A-1(L) is a Myoviridae cyanophage isolated in 1970s9 that specifically infects the model cyanobacterium Anabaena sp. PCC 7120. Using cryo-electron microscopy (cryo-EM), we solved the structure of A-1(L) tail machine, which consists of three parts: a 205-Å-long neck, a 1045-Å-long contractile tail with a complicated baseplate, and six pairs of tail fibers. The dodecameric gp2 portal, the pentadecameric gp5 and the hexameric gp7 sequentially constitute the neck of A-1(L), to which five neck fibers are attached. The long and contractile tail of A-1(L) contains 24 rings of gp10 hexamers that form the tube, surrounded by the sheath of 24 helically stacked gp9 hexamers.

Moreover, docking of tail to the neck is accomplished via direct interactions: Loopβ4-β5 (residues Gly55-Thr65) of one gp7 subunit and antiparallel β4′-β5′ hairpin of neighboring subunit interact with Loopα1-β1 (residues Ile15-Val34) and Loopβ5-β6 (residues Leu135-Trp152) of one terminator/gp8 subunit, respectively. In detail, the ring formed by Loopα4-α5 (residues Ile83-Tyr99) of 15 gp5 subunits is hooked by six long α1 helices (residues Met1-Leu25) at the N-terminus of gp7, whereas Loopα1-α2 (residues Leu20-Glu30) of three gp5 subunits tightly interact with the Loopβ5-β6 (residues Thr70-Lys75) of trimeric gp82N. In contrast to the initiation with two separate proteins, the termination of the tube and sheath is fulfilled by a same terminator. Each terminator subunit simultaneously interacts with two tube subunits via Loopβ3-β4 (residues Thr58-Gln71) and β5 (residues Thr125-Leu135), and one sheath subunit via a protruding β7-β8 hairpin (residues Asn202-Ile240), which disrupts the inter-ring interfaces of the tube and sheath, and eventually terminates the extension of tail. Notably, the A-1(L) terminator is structurally different from the previously reported ones in the tailed phages and eCISs. The tube and sheath start from the tube initiator/hexameric gp18 and sheath initiator/hexameric gp30, respectively, but both stop at the same terminator/hexameric gp8. In addition, structural analysis suggested that all pairwise interfaces are complementary in shape and electrostatic potential, enabling the interlocked assembly of the symmetry-mismatched A-1(L) neck.

>[6x]MLYSNLINVKQKVISIREKLGDPRLKSLVFEYPAGQLFRVTPKLKVSMVPKNMIGLPLDSKSNITISADDYYITDVSRNVPEAAFRTRAWLDPVINDSGVIVSGINCRCHVINDKSGLSYDLILRKEREVRV;>[6x]MTKPSLISAKILQHINSIVWLQSKGIQEPLKPDVIVNNVAYPPNVIAEKPVTNIEVITNSSMIENTGGVRQFLCKAVFEYTIVWVFSREVYKTYHQIPRSQIQDLLVFCQQFVISAYQGIDPDITNIDLKPSQVLVKPTEDVNSDVSNSSSWSVVADLRFMIEFLTSLDEFLPIDFNKIQPPTWELLDDLDPIVPEQPFTLNGLIISLNKSELPKVRADESDTYQLEEILYIPPTIEDQI>[12x]MDKLEIGFEVFTFPREEEITIEVIEEFMSLHSKQQPRYERLMKMYKGDAAIFARKAKEPHKPDNRLNVNYAKYITDTFSGFFNGIPSKKNHKNDVVSDAINNFDNEQDMQDEEAELVKLACVYGHAFELMYQDEETKTNVKHNSPEDMFIVYDDTVSQKPLFAVRYGLDREGELCGTLYTEDVDVTLIGKNGTMIFGEESENVY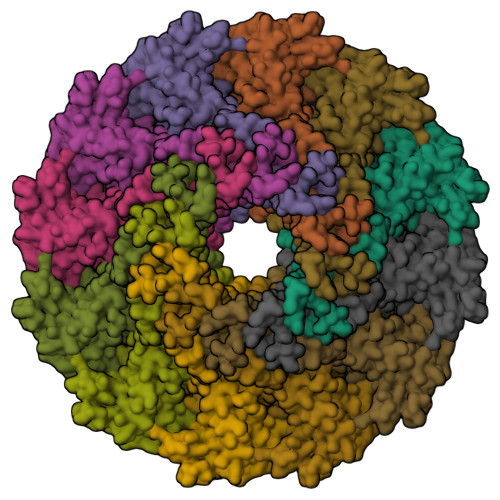NDLAVTEFIFNEERMGIYETVTALIDSYDKAISEKTNDVDYFSDSYLKVVGAMLSPEMIEKIRDTRVINVPEPPHDVSVDIGFLDKPDSDSQTENLLDRIDKHIYQIAMVANISDESFGSSSGVALAYKLQPMSNLAAAFERKFQAALTQRYKMFMSLLTNVSANLSNEWRGIEFRFTRNIPKNVLEEAQTAVQLATIASQETTLSVLSVVPDVRAEMDRIHSERKDDINLLDYQQEVPEKETVEVVEKEDS>MGSSHHHHHHSSGRENLYFQGHVEPGVTDRIGQMILEMFRTGMCLFSVRSPGGVAELYGGEARKVEITGTSLTIEREDWHLHCKLETVETVVFDLSPKDNGGIRMAVVFRDK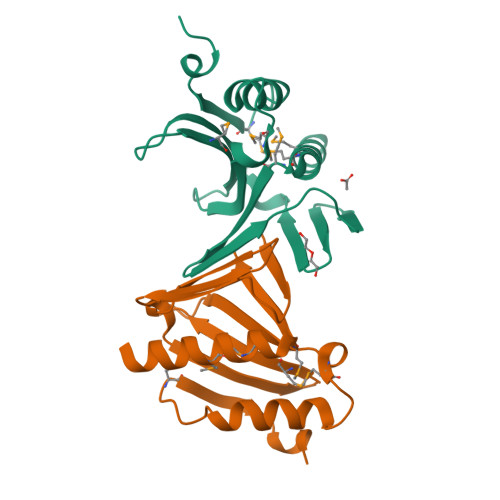HQAPVLRAAWLPRLMPETPSPPEQFWAFTQRYIDLPMVVDARNRQLVFPGSGQGGFTEGS[4x]>[3x]MLEANVYDNFNPNYYNISDFSMPNGKKEKRGLPIPKARCQVINYELWETGYLYTSSATLTVSVEVGDIVQILFPEVVPIEEALGKKKKLNLDMVYLVTDVDESNKATLKNYFWAMIESLDVPNAITKTTNFAIIDYLIDPNKNNLMSYGYFFNSSIFAGKATINRKAETSSAHDVAKRIFSKVQFQPTTTIQHAPSETDPRNLLFINFASRNWNRKRITTRVDIKQSVTMDTETIVERSAYNFAVVFVKNKATDDYTDPPKMYIAKNNGDVIDYSTYHGDGTDLPDVRTAKTLFYDRDDHGNPPELSTIKVEISPSTIVTRLIFNQNELLPLYVNDLVDIWYEGKLYSGYIADRVKTEFNDRLIFVESGDKPNVI;>[12x]MVRQYKIHTNLDGTDDKVWDVTNGKVRFYQPSNLGLQSTNNIWQSNGIGVMGTRSITQPQIEFKLETFGESLEENYQLMKDFVNDILSKKFVTLEYQTEIFQVYADLALADVTKTEGYGKNGTFSEKITFDIITKWYTYENLTFDKIQNGKVIAGMSKIYGGTAPGNYKYIKGTSYTYYGESDIDRLSRWDIKEEIFSFMGILYPKLPKTPAGVRFLDDIGNEYTAIVFKTEQVQDYILINTDVNDETYQGWKGTTALNLFPVMDFERYRTRIIEKGQMELINLSKAEFKIKRKADFV;>MTIKNFTFFSPNSTEFPVGSNNDGKLYMMLTGMDYRTIRRKDWSSPLNTALNVQYTNTSIIAGGRYFELLNETVALKGDSVNYIHANIDLTQTANPVSLSAETANNSNGVDINNGSGVLKVCFDIVTTSGTGVTSTKPIVQTSTLDSISVNDMTVSGSIDVPVQTLTVEAGNGLQLQLTKKNNDLVIVRFFGSVSNIQKGWNMSGTWVDRPFRPAAVQSLVGHFAGRDTSFHIDINPNGSITWWGANIDKTPIATRGNGSYFIK[18x]

Virulent phages belonging to the newly created Skunavirus genus (previously 936) are by far the most predominant in dairy factories and they currently belong to the Siphoviridae family (double-stranded DNA genome and non-contractile tail) of the Caudovirales order. Phage p2 is the model phage for this viral genus and it infects L. lactis MG1363, a laboratory strain used in many studies on Gram-positive bacteria. Of interest here, phage p2 uses a multi-protein baseplate at the tip of its tail to bind to its cell wall polysaccharide (CWPS) receptor at the host cell surface. Here, we present further structural analyzes of the phage p2 baseplate, proposing a topological model of the baseplate resting state, and interpreting a new nsEM structure of the virion, in its active conformation.

However, when Ca2+ (or Sr2+) was added to the purified baseplate complex, the baseplate exhibited a different conformation in which the receptor-binding domains point downwards in the direction opposite to the capsid. In addition, the Tal trimer adopted an open conformation instead of a closed one in the purified baseplate-VHH5 complex. In both baseplate conformations, an extension of the Dit galectin domain, the “arm”, holds the RBPs by inserting its “hand” within the trimeric RBP “shoulder” domain. In this context, it was proposed that the structure obtained in the presence of Ca2+ was an actived form of the phage baseplate. It was also suggested that the baseplate transition from resting to activated state could be the trigger for Tal opening and subsequent release of the tail tape measure protein (TMP), followed by DNA ejection. However, we were unable to obtain this baseplate activated state in p2 virions, despite many attempts, which included the addition of divalent cations (Ca2+, Sr2+), hampering somewhat the validity of the suggested activation mechanism.EfeUOB/M has been characterised in Pseudomonas syringae pathovar. syringae as a novel type of ferrous-iron transporter, consisting of an inner-membrane protein (EfeUPsy) and three periplasmic proteins (EfeOPsy, EfeMPsy and EfeBPsy). EfeMPsy is an ‘M75-only’ EfeO-like protein with a C-terminal peptidase-M75 domain (EfeOII/EfeM family). Here we report the X-ray structure determination and bioanalytical characterisation of EfeMPsy from Pseudomonas syringae pv. syringae B728a; an EfeM family member that shares ~ 60% sequence identity with EfeO of E. coli K-12 in an effort to understand the role of this protein family member in the EfeUOB/M systems in bacteria. The work reported here introduces EfeMPsy as the best candidate to mark the beginning of the journey for a more detailed understanding of the periplasmic components, EfeO (EfeOI family) and EfeM (EfeOII family) and thereby offers support for the suggestion that these proteins contribute to iron transport in the EfeUOB(M) system, acting as periplasmic iron-binding proteins.

Herein, we report a structure solution of the apo form of EfeMPsy by molecular replacement. The refined structure of EfeMPsy consists of two identical EfeMPsy monomers (chain A, residues A35-A285, and chain B, residues B35-B285) in the asymmetric unit. Close examination of the overall structure shows that EfeMPsy is composed of two major α-helical bundles designated as ‘B1’ and ‘B2’. A flexible loop (residues 162–165, highlighted as ‘IDH’ in Fig. 1a) separates the B1 (residues 36–161) and B2 bundles (residues 166–285). Comparison of the folds (EfeMPsy vs pSBPs) suggests that some of the key structural characteristics of pSBPs are retained by EfeMPsy; the presence of two discrete domains linked by a hinge region, and the presence of an inter-domain ligand-binding cleft. Moreover, the inter-domain hinge region of EfeMPsy is smaller, consisting of only four residues which may reflect the relative size of ligand, in this case a metal ion, and potentially the lack of necessity to undergo any substantial opening/closing of the cleft to facilitate ligand binding. In this work, a closer examination of the structure of EfeMPsy has revealed two potential metal binding sites. The metal binding cleft, Site III, is nestled in between the two alpha helix bundles B1 and B2. Based on these observations, arising from the crystal structure, up to five residues (Tyr82, His126, Glu129, Glu189 and Asp190) can be considered potential metal ligands at Site III.Assessment of the structure for other potential metal binding sites, suggests a potential second metal binding site for these EfeO/EfeM family of proteins.

>MTYPLLTRKTLMKKTPLALLLTLGLLQTPLAAFAATAPLDLVGPVSDYKIYVTENIEELVSHTQKFTDAVKKGDIATAKKLYAPTRVYYESVEPIAELFSDLDASIDSRVDDHEQGVAAEDFTGFHRLEYALFSQNTTKDQGPIADKLLSDVKDLEKRVADLTFPPEKVVGGAAALLEEVAATKISGEEDRYSHTDLYDFQGNIDGAKKIVDLFRPQIEQQDKAFSSKVDKNFATVDKILAKYKTKDGGFETYDKVKENDRKALVGPVNTLAEDLSTLRGKLGLN[2x]L-XYLULOSE 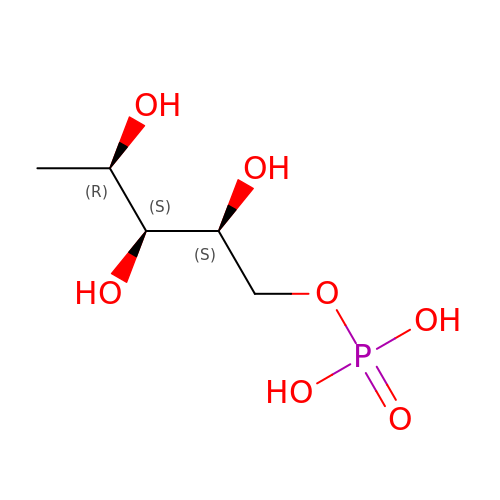5-PHOSPHATE | C5 H13 O7 P | YPXGTKHZRCDZTL-WISUUJSJSA-N> AANSVVAYGRWPEYLRD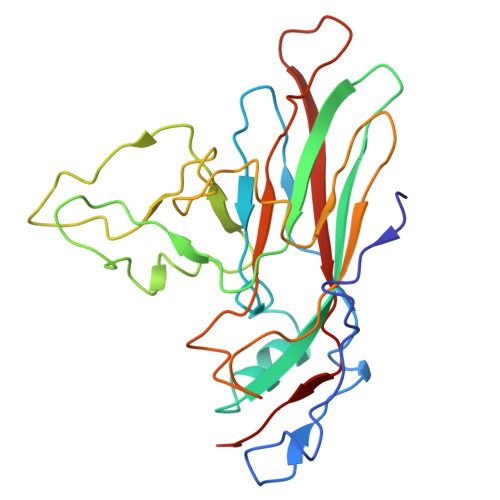SEANPVDQPTEPDVAACRFYTLDTVSWTKESRGWWWKLPDALRDMGLFGQNMYYHYLGRSGYTVHVQCNASKFHQGALGVFAVPEMCLAGDSNTTTMHTSYQNANPGEKGGTFTGTFTPDNNQTSPARRFCPVDYLLGNGTLLGNAFVFPHQIINLRTNNCATLVLPYVNSLSIDSMVKHNNWGIAILPLAPLNFASESSPEIPITLTIAPMCCEFNGLR> GPQIASMSATALLQKAAQMGSKRSSSSSSNSKTFGLMT;> GPMVAMFQEDNGTSSVASSPLQVFSTMSLNRPTLLASSSPFHCLKDLKPEERGLYLIHLLLTCANHVASGSLQNANAALEQLSHLASPDGDTMQRIAAYFTEALANRILKSWPGLYKALNATQT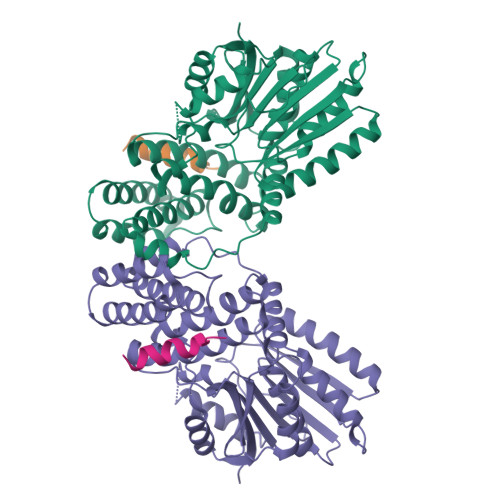RTNNVSEEIHVRRLFFEMFPILKVSYLLTNRAILEAMEGEKMVHVIDLDASEPAQWLALLQAFNSRPEGPPHLRITGVHHQKEVLEQMAHRLIEEAEKLDIPFQFNPVVSRLDCLNVEQLRVKTGEALAVSSVLQLHTFLASDDDLMENDMSNNNGYSPSGDSASSLPLPSSGRTDSFLNAIWGLSPKVMVVTEQDSDHNGSTLMERLLESLYTYAALFDCLETKVPRTSQDRIKVEKMLFGEEIKNIISCEGFERRERHEKLEKWSQRIDLAGFGNVPLSYYAMLQARRLLQGCGFDGYRIKEESGCAVICWQDRPLYSVSAWRCRK>[24x]RSYEQMETDGERQNATEIRASVGKMIDGIGRFYIQMCTELKLSDYEGRLIQNSLTIERMVLSAFDERRNKYLEEHPSAGKDPKKTGGPIYRRVDGKWRRELILYDKEEIRRIWRQANNGDDATAGLTHMMIWHSNLNDATYQRTRALVRTGMDPRMCSLMQGSTLPRRSGAAGAAVKGVGTMVMELIRMIKRGINDRNFWRGENGRRTRIAYERMCNI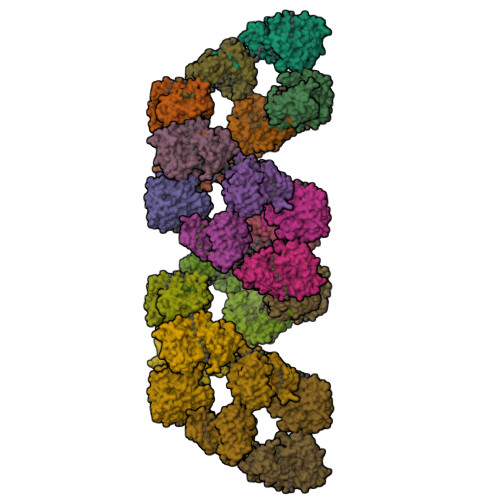LKGKFQTAAQRTMVDQVRESRNPGNAEFEDLIFLARSALILRGSVAHKSCLPACVYGSAVASGYDFEREGYSLVGIDPFRLLQNSQVYSLIRPNENPAHKSQLVWMACHSAAFEDLRVSSFIRGTKVVPRGKLSTRGVQIASNENMETMESSTLELRSRYWAIRTRSGGNTNQQRASSGQISIQPTFSVQRNLPFDRPTIMAAFTGNTEGRTSDMRTEIIRLMESARPEDVSFQGRGVFELSDEKATSPIVPSFDMSNEGSYFFGDNAEEYDNLEHHHHHH> XXXXXXXXXXXXXXXXXXXXXXXXXXXXXXXXXXXXXXXXXXXXXXXXXXXXXXXXXXXXXXXXXXXKLTLGLSILFMVEAAEFTVPKKDLDSLCYLLIPSAGSPEALHSDLSPVLRIRQRWRIYLTNLCLRCIDERCDRWLGILPLLHTCMQKSPPKKNSKSQPEDTWAGLEGISFSEFRDKAPTRSQPLQFMQSKMALLRVDEYLFRSWLSVVPLESLSSYLENSIDYLSDVPVRVLDCLQGISYRLPGLRKISNQNMKKDVENVFKMLMHLVDIYQHRIFGENLLQIYLTECLTLHETVCNITANHQFFEIPALSAELICKLLELSPPGHTDEGLPEKSYEDLVTSTLQEALATTRNWLRSLFKSRMLSISSAYVRLTYSEEMAVWRRLVEIGFPEKHGWKGSLLGDMEGRLKQEPPRLQISFFCSSQCRDGGLHDSVSRSFEKCVIEAVSSACQSQTSVLEGLSCQDLQKFGTLLSAVITKSWPVHNGEPVFDVDEIFKYLLKWPDVRQLFELCGTNEKIIDNITEEGRQLMATAESVFQKVAGELENGTIVVGQLELILEHQSQFLDIWNLNRRRLPSQEKACDVRSLLKRRRDDLLFLKQEKRYVESLLRQLGRVKHLVQVDFGNIEIIHSQDLSNKKLNEAVIKLPNSSSYKRETHYCLSPDIREMASKLDSLKDSHIFQDFWQETAESLNTLDKDPRELKVSLPEVLEYLYNPCYDNFYTLYENLKSGKITFAEVDAIFKDFVDKYDELKNDLKFMCTMNPQDQKGWISERVGQIKEYHTLHQAVSSAKVILQVRRALGVTGDFSVLNPLLNFADSFEDFGNEKLDQISPQFIKAKQLLQDISEPRQRCLEELARQTELVAWLHKALEDINELKVFVDLASISAGENDIDVDRVACFHDAVQGYASLLYKMDERTNFSDFMNHLQELWRALDNDQHLPDKLKDSARNLEWLKTVKESHGSVELSSLSLATAINSRGVYVIEAPKDGQKISPDTVLRLLLPDGHGYPEALRTYSTEELKELLNKLMLMSGKKDHNSNTEVEKFSEVFSNMQRLVHVFIKLHCAGNMLFRTWTAKVYCCPDGGIFMNFGLELLSQLTEKGDVIQLLGALCRQMEDFLDNWKTVVAQKRAEHFYLNFYTAEQLVYLSSELRKPRPSEAALMMLSFIKGKCTVQDLVQATSACESKADRYCLREVMKKLPQQLLSEPSLMGKLQVIMMQSLVYMSAFLPHCLDLDALGRCLAHLATMGGTPVERPLPKGLQAGQPNLILCGHSEVLPAALAIYMQAPRQPLPTFDEVLLCTPATTIEEVELLLRRCLTSGSQGHKVYSLLFADQLSYEVGCQAEEFFQSLCTRAHREDYQLVILCDAAREHCYIPSTFSQYKVPLVPQAPLPNIQAYLQSHYQVPKRLLSAATVFRDGLCVGIVTSERAGVGKSLYVNTLHTKLKAKLRDETVPLKIIRLTEPHLDENQVLSALLPFLKEKYQKMPVIFHIDISTSVQTGIPIFLFKLLILQYLMDINGKIWRRSPGHLYLVEIPQGLSVQPKRSSKLNARAPLFKFLDLFPKVTCRPPKEVIDMELTPERSHTDPAMDPVEFCSEAFQRPYQYLKRFHQQQNLDTFQYEKGSVEGSPEECLQHFLIYCGLINPSWSELRNFAWFLNCQLKDCEASIFCKSAFTGDTLRGFKNFVVTFMILMARDFATPTLHTSDQSPGRQSVTIGEVVEEDLAPFSLRKRWESEPHPYVFFNGDHMTMTFIGFHLETNNNGYVDAINPSNGKVIKKDVMTKELFDGLRLQRVPFNIDFDNLPRYEKLERLCLALGIEWPIDPDETYELTTDNMLKILAIEMRFRCGIPVIIMGETGCGKTRLIKFLSDLKRGSVEAETMKLVKVHGGTTPSMIYSKVKEAERTAFSNKAQHKLDTILFFDEANTTEAVSCIKEILCDRTVDGEHLHEDSGLHIIAACNPYRKHSQEMILRLESAGLGYRVSAEETADRLGSIPLRQLVYRVHALPPSLIPLVWDFGQLNDSAEKLYIQQIVQRLVDSVSVNPSETCVIADVLSASQMFMRKRENECGFVSLRDVERCVKVFRWFHDHSDMLLKELDKFLHESSDSTHTFERDPVLWSLVMAIGVCYHASLEEKASYRTAIARCFPKPYNSSRAILDEVTHVQDLFLRGAPIRTNIARNLALKENVFMMVICIELKIPLFLVGKPGSSKSLAKIIVADAMQGQAAFSELFRCLKQVHLVSFQCSPHSTPQGIISTFKQCARFQQGKDLGQYVSVVVLDEVGLAEDSPKMPLKTLHPLLEDGCIEDDPAPYKKVGFVGISNWALDPAKMNRGIFVSRGSPNEKELIESAEGICSSDRLVQDKIRGYFAPFAKAYETVCQKQDKEFFGLRDYYSLIKMVFAKAKASKRGLSPQDITHAVLRNFSGKDNIQALSIFTASLPEARYKEEVSTVELIKQNIYPGPQASSRGLDGAESRYLLVLTRNYVALQILQQTFFEGQQPEIIFGSSFPQDQEYTQICRNINRVKICMETGKMVVLLNLQNLYESLYDALNQYYVYLGGQKYVDLGLGTHRVKCRVHTAFRLIVIEEKDVVYKQFPVPLINRLEKHYLDMNTVLQPWQKSIVQELQQWAHEFADVKADQFIARHKYSPADVFIGYHSDACASVVLQAVERQGCRDLTEELYRKVSEEARSILLDCATPDAVVRLSGSSLGSFTAKQLSQEYYYAQQHNSFVDFLQAHLRMTHHECRAVFTEITTFSRLLTGNDCDVLASELRGLASKPVVLSLQQYDTEYSFLKDVRSWLTNPGKRKVLVIQADFDDGTRSAQLVASAKYTAINEINKTQGTKDFVFVYFVTKLSRMGSGTSYVGFHGGLWRSVHIDDLRRSTIMASDVTKLQNVTISQLFKPEDKPEQEEMEIETSQSKELAEEQMEVEDSEEMKKASDPRSCDCSQFLDTTRLVQSCVQGAVGMLRDQNESCARNMRRVTILLDLLNEDNTRNASFLRESKMRLHVLLNKQEENQVRSLKEWVTREAANQDALQEAGTFRHTLWKRVQDVVTPILASMIAHIDRDGNLELLAQPDSPAWVQDLWMFIYSDIKFLN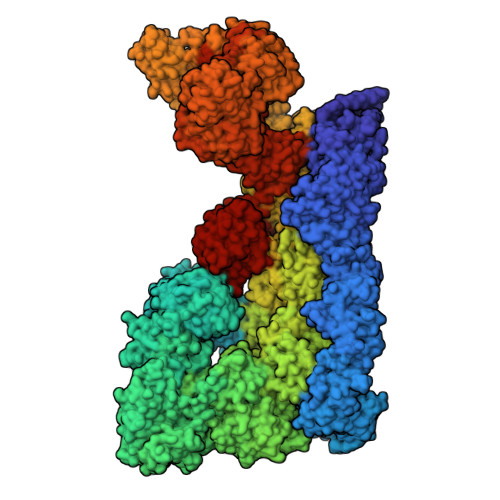ISLVLNNTRSNSEMSFILVQSHMNLLKDAYNAVPFSWRIRDYLEELWVQAQYITDTEGLSKKFVEIFQKTPLGVFLAQFPVAQQQKLLQSYLKDFLLLTMKVSSREELMFLQMALWSCLRELQEASGTPDETYKFPLSLPWVHLAFQHFRTRLQNFSRILTIHPQVLSSLSQAAEKHSLAGCEMTLDAFAAMACAEMLKGDLLKPSPKAWLQLVKNLSTPLELVCSEGYLCDSGSMTRSVIQEVRALWNRIFSIALFVEHVLLGTESHIPELSPLVTTYVSLLDKCLEEDSNLKTCRPFVAVMTTLCDCKDKASKKFSRFGIQPCFICHGDAQDPVCLPCDHVYCLRCIQTWLIPGQMMCPYCLTDLPDKFSPTVSQDHRKAIEKHAQFRHMCNSFFVDLVSTMCFKDNTPPEKSVIDTLLSLLFVQKELLRDASQKHREHTKSLSPFDDVVDQTPVIRSVLLKLLLKYSFHEVKDYIQNYLTQLEKKAFLTEDKTELYLLFISCLEDSVHQKTSAGCRNLEQVLREEGHFLRTYSPGLQGQEPVRIASVEYLQEVARVRLCLDLAADFLSELQEGSELAEDKRRFLKHVEEFCTRVNNDWHRVYLVRKLSSQRGMEFVQSFSKQGHPCQWVFPRKVIAQQKDHVSLMDRYLVHGNEYKAVRDATAKAVLECKTLDIGNALMACRSPKPQQTAYLLLALYTEVAALYRSPNGSLHPEAKQLEAVNKFIKESKILSDPNIRCFARSLVDNTLPLLKIRSANSILKGTVTEMAVHVATILLCGHNQILKPLRNLAFYPVNMANAFLPTMPEDLLVHARTWRGLENVTWYTCPRGHPCSVGECGRPMQESTCLDCGLPVGGLNHTPHEGFSAIRNNEDRTQTGHVLGSPQSSGVAEVSDRGQSPVVFILTRLLTHLAMLVGATHNPQALTVIIKPWVQDPQGFLQQHIQRDLEQLTKMLGRSADETIHVVHLILSSLLRVQSHGVLNFNAELSTKGCRNNWEKHFETLLLRELKHLDKNLPAINALISQDERISSNPVTKIIYGDPATFLPHLPQKSIIHCSKIWSCRRKITVEYLQHIVEQKNGKETVPVLWHFLQKEAELRLVKFLPEILALQRDLVKQFQNVSRVEYSSIRGFIHSHSSDGLRKLLHDRITIFLSTWNALRRSLETNGEIKLPKDYCCSDLDLDAEFEVILPRRQGLGLCGTALVSYLISLHNNMVYTVQKFSNEDNSYSVDISEVADLHVISYEVERDLNPLILSNCQYQVQQGGETSQEFDLEKIQRQISSRFLQGKPRLTLKGIPTLVYRRDWNYEHLFMDIKNKMAQSSLPNLAISTISGQLQSYSDACEALSIIEITLGFLSTAGGDPGMDLNVYIEEVLRMCDQTAQVLKAFSRCQLRHIIALWQFLSAHKSEQRLRLNKELFREIDVQYKEELSTQHQRLLGTFLNEAGLDAFLLELHEMIVLKLKGPRAANSFNPNWSLKDTLVSYMETKDSDILSEVESQFPEEILMSSCISVWKIAATRKWDRQSRGGGHHHHHHHHHH> SASGVDDRDLLLAPKWISFLSLSSFLKQKLLSLLRQIRELRLTTTVYPPQDKLMWWSHCCDPEDIKVVILGQDPYHKGQATGLAFSVDPQCQVPPSLRSIFRELEASVPNFSTPSHGCLDSWARQGVLLLNTVLTVEKGRAGSHEGLGWDWFTSFIISSISSKLEHCVFLLWGRKAIDRTPLINAQKHLVLTAQHPSPLASLGGRHSRWPRFQGCNHFNLANDYLTRHRRETVDWGLLEQ

Efficient γ-herpesvirus lytic phase replication requires a virally encoded UNG-type uracil-DNA glycosylase as a structural element of the viral replisome. Uniquely, γ-herpesvirus UNGs carry a seven or eight residue insertion of variable sequence in the otherwise highly conserved minor-groove DNA binding loop. The UNG leucine loop is a conserved structural feature which is responsible for widening the DNA minor groove and flipping pyrimidines out of the base stack and, in the case of uracil, into the UNG active site for catalysis. kUNG, in common with other known UNGs, comprises a single C-terminal globular domain made up of a four-stranded parallel β-sheet flanked by six α-helices, with an additional left-handed coil of three helices at the N-terminus.

The structure of kUNG in its apo form was solved in two different crystal forms. The disc-shaped structure of the leucine loop extension centred on the side chain of Q212 was not observed in the two unbound kUNG structures. Taken together, the unbound kUNG structures suggest that the leucine loop extension is highly flexible in solution. However, the absence of electron density for the leucine loop insertion in the apo kUNG C2 crystal form, and partial ordering of the leucine loop along with significant crystal contacts in the P21 crystal form indicate that the leucine loop is very likely highly mobile in solution. Mutagenesis suggests a model in which the kUNG loop is pinned outside the DNA-binding cleft until DNA docking promotes rigid structuring of the loop and duplex nucleotide flipping, a novel observation for UNGs.5'-O-[(S)-hydroxy{[(S)-hydroxy{[(1-hydroxy-2,2,5,5-tetramethyl-2,5-dihydro-1H-pyrrol-3-yl)methyl]disulfanyl}phosphoryl]oxy}phosphoryl]adenosine | C19 H30 N6 O10 P2 S2 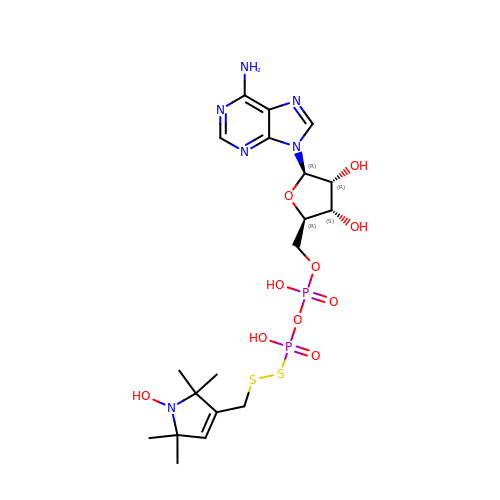| FXTBVPRAZDKBSQ-LSCFUAHRSA-N> GAFLDKPKMEKHNAQGQGNGLRYGLSSMQGWRVEMEDAHTAVIGLPSGLESWSFFAVYDGHAGSQVAKYCCEHLLDHITNNQDFKGSAGAPSVENVKNGIRTGFLEIDEHMRVMSEKKHGADRSGSTAVGVLISPQHTYFINCGDSRGLLCRNRKVHFFTQDHKPSNPLEKERIQNAGGSVMIQRVNGSLAVSRALGDFDYKCVHGKGPTEQLVSPEPEVHDIERSEEDDQFIILACDGIWDVMGNEELCDFVRSRLEVTDDLEKVCNEVVDTCLYKGSRDNMSVILICFPNAPKVSPEAVKKEAELDKYLECRVEEIIKKQGEGVPDLVHVMRTLASENIPSLPPGGELASKRNVIEAVYNRLNP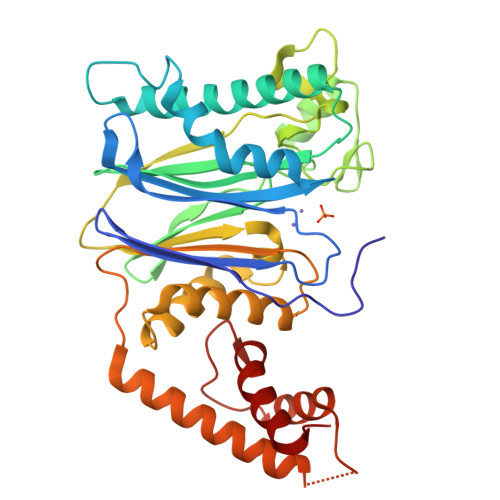Y> GPVEDVITAAIGRVADTVGTGPTNSEAIPALTAAETGHTSQVVPGDTMQTRHVKNYHSRSESTVENFLCRSACVYFTEYKNSGSKRYAEWVVTTRQAAQLRRKLEFFTYIRFDLELTFVITSTQQPSTTQNQDAQILTHQIMYVPPGGPVPDKVDSYVWQTSTNPSVFWTEGNAPPRMSIPFLSIGNAYSNFYDGWSEFSRNGVYGINTLNNMGTLYARHVNTGSTGPIKSTIRIYFKPKHVKAWIPRPPRLCQYEKAKNVNFQPSGVTTTRQSIT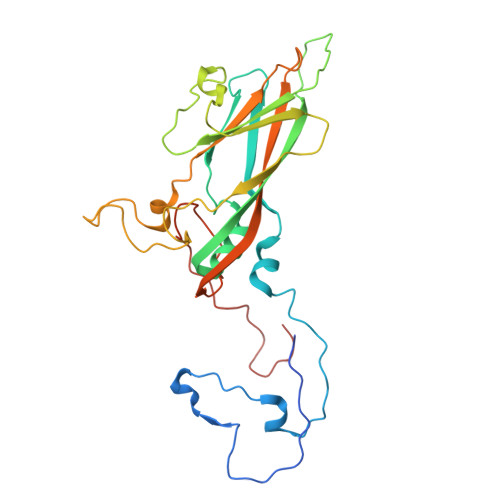TMTNTGAF>GPLESSHHRSTQQLQTKVSELETANRELIDKKYKSDSTIRDLKAKMTSLEEECQRSKQQVLSLRRENSALDSECHEKERLMNQLQTRVAVLEQEIKDKDQLVLR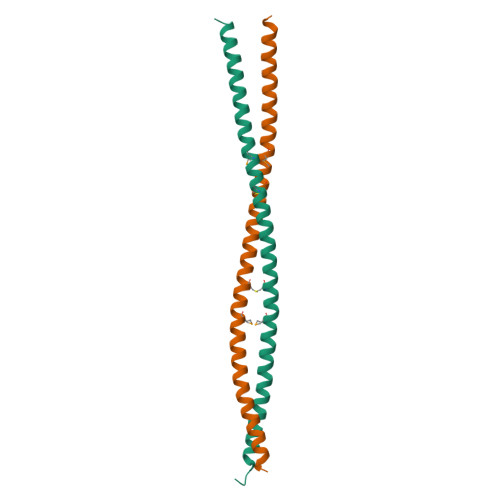TKEVLEATQQQKNS[4x]>[6x]LDKVYQMKSKPRGYCLIINNHNFAKAREKVPKLHSIRDRNGTHLDAGALTTTFEELHFEIKPHHDCTVEQIYEILKIYQLMDHSNMDCFICCILSHGDKGIIYGTDGQEAPIYELTSQ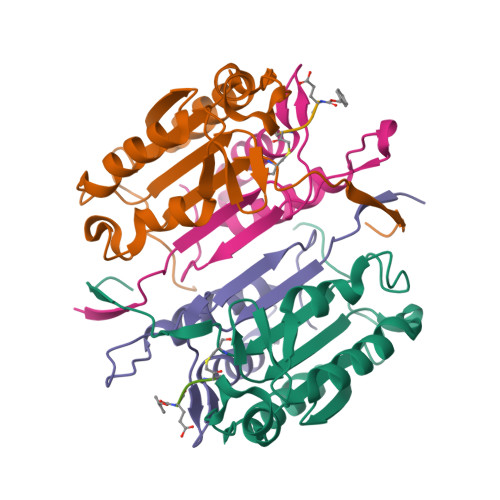FTGLKCPSLAGKPKVFFIQACQGDNYQKGIPVETD;>[6x]TRYIPDEADFLLGMATVNNCVSYRNPAEGTWYIQSLCQSLRERCPRGDDILTILTEVNYEVSNKDDKKNMGKQMPQPTFTLRKKLVFP> MKPYYVTTAIAYPNAAPHVGHAYEYIATDAIARFKRLDRYDVRFLTGTDEHGLKVAQAAAAAGVPTAALARRNSDVFQRMQEALNISFDRFIRTTDADHHEASKELWRRMSAAGDIYLDNYSGWYSVRDERFFVESETQLVDGTRLTVETGTPVTWTEEQTYFFRLSAYTDKLLAHYHANPDFIAPETRRNEVISFVSGGLDDLSISRTSFDWGVQVPEHPDHVMYVWVDALTNYLTGAGFPDTDSELFRRYWPADLHMIGKDIIRFHAVYWPAFLMSAGIELPRRIFAHGFLHNRGEKMSKS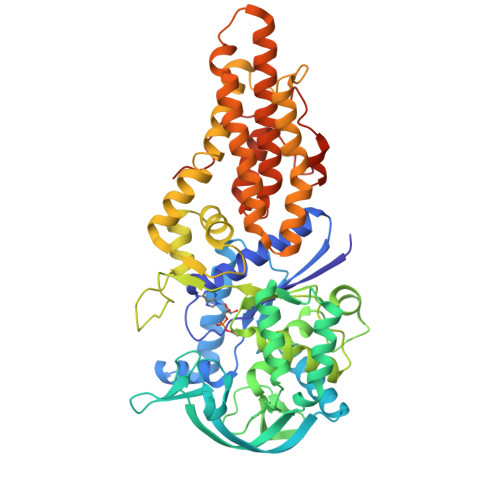VGNIVDPVALAEALGVDQVRYFLLREVPFGQDGSYSDEAIVTRINTDLANELGNLAQRSLSMVAKNLDGRVPNPGEFADADAALLATADGLLERVRGHFDAQAMHLALEAIWLMLGDANKYFSVQQPWVLRKSESEADQARFRTTLYVTCEVVRIAALLIQPVMPESAGKILDLLGQAPNQRSFAAVGVRLTPGTALPPPTGVFPRYQPPQPPEGK>GQDRLDAPPPPAPPLLRWAGPVGVSWGLRAAAPGGPVPRAGRWRRGAPAEDQDCGRLPDFIAKLTNNTHQHVFDDLSGSVSLSWVGDSTGVILVLTTFQVPLVIVSFGQSKLYRSEDYGKNFKDITNLINNTFIRTEFGMAIGPENSGKVILTAEVSGGSRGGRVFRSSDFAKNFVQTDLPFHPLTQMMYSPQNSDYLLALSTENGLWVSKNFGEKWEEIHKAVCLAKWGPNNIIFFTTHVNGSCKADLGALELWRTSDLGKTFKTIGVKIYSFGLGGRFLFASVMADKDTTRRIHVSTDQGDTWSMAQLPSVGQEQFYSILAANEDMVFMHVDEPGDTGFGTIFTSDDRGIVYSKSLDRHLYTTTGGETDFTNVTSLRGVYITSTLSEDNSIQSMITFDQGGRWEHLRKPENSKCDATAKNKNECSLHIHASYSISQKLNVPMAPLSEPNAVGIVIAHGSVGDAISVMVPDVYISDDGGYSWAKMLEGPHYYTILDSGGIIVAIEHSNRPINVIKFSTDEGQCWQSYVFTQEPIYFTGLASEPGARSMNISIWGFTESFITR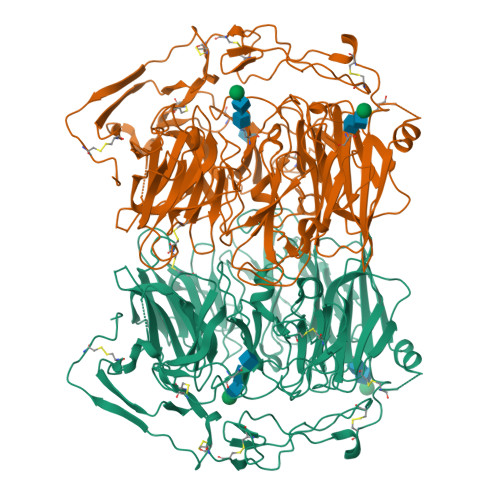QWVSYTVDFKDILERNCEEDDYTTWLAHSTDPGDYKDGCILGYKEQFLRLRKSSVCQNGRDYVVAKQPSVCPCSLEDFLCDFGYFRPENASECVEQPELKGHELEFCLYGKEEHLTTNGYRKIPGDKCQGGMNPAREVKDLKKKCTSNFLNPTKQNSKSNAAAHHHHHH[4x]> MKEFYLTVEQIGDSIFERYIDSNGRERTREVEYKPSLFAHCPESQATKYFDIYGKPCTRKLFANMRDASQWIKRMEDIGLEALGMDDFKLAYLSDTYNYEIKYDHTKIRVANFDIEVTSPDGFPEPSQAKHPIDAITHYDSIDDRFYVFDLLNSPYGNVEEWSIEIAAKLQEQGGDEVPSEIIDKIIYMPFDNEKELLMEYLNFWQQKTPVILTGWNVESFAIPYVYNRIKNIFGESTAKRLSPHRKTRVKVIENMYGSREIITLFGISVLDYIDLYKKFSFTNQPSYSLDYISEFELNVGKLKYDGPISKLRESNHQRYISYNIIAVYRVLQIDAKRQFINLSLDMGYYAKIQIQSVFSPIKTWDAIIFNSLKEQNKVIPQGRSHPVQPYPGAFVKEPIPN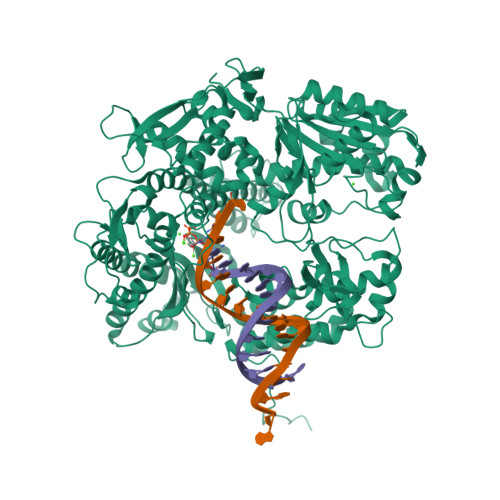RYKYVMSFDLTSLYPSIIRQVNISPETIAGTFKVAPLHDYINAVAERPSDVYSCSPNGMMYYKDRDGVVPTEITKVFNQRKEHKGYMLAAQRNGEIIKEALHNPNLSVDEPLDVDYRFDFSDEIKEKIKKLSAKSLNEMLFRAQRTEVAGMTAQINRKLLINSLAGALGNVWFRYYDLRNATAITTFGQMALQWIERKVNEYLNEVCGTEGEAFVLYGDTDSIYVSADKIIDKVGESKFRDTNHWVDFLDKFARERMEPAIDRGFREMCEYMNNKQHLMFMDREAIAGPPLGSKGIGGFWTGKKRYALNVWDMEGTRYAEPKLKIMGLETQKSSTPKAVQKALKECIRRMLQEGEESLQEYFKEFEKEFRQLNYISIASVSSANNIAKYDVGGFPGPKCPFHIRGILTYNRAIKGNIDAPQVVEGEKVYVLPLREGNPFGDKCIAWPSGTEITDLIKDDVLHWMDYTVLLEKTFIKPLEGFTSAAKLDYEKKASLFDMFDF> GG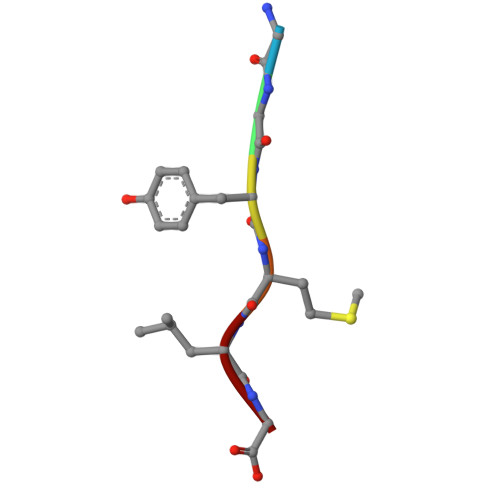YMLG alpha-L-xylopyranose | C5 H10 O5 | 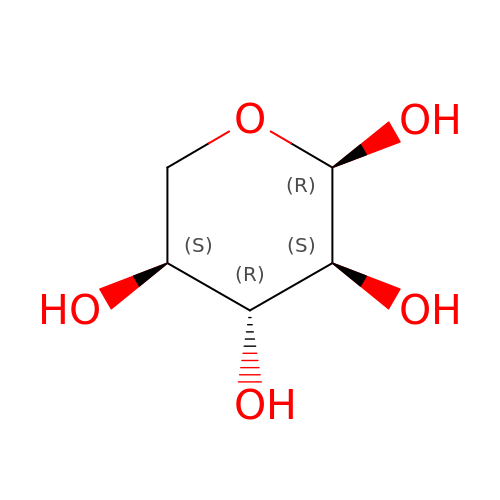SRBFZHDQGSBBOR-SKNVOMKLSA-N> SMDMPVERILEAELAVEPKTETYVEANMGLNPSSPN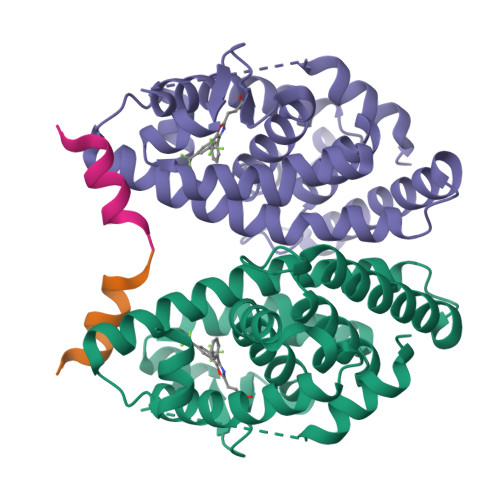DPVTNICQAADKQLFTLVEWAKRIPHFSELPLDDQVILLRAGWNELLIASFSHRSIAVKDGILLATGLHVHRNSAHSAGVGAIFDRVLTELVSKMRDMQMDKTELGCLRAIVLFNPDSKGLSNPAEVEALREKVYASLEAYCKHKYPEQPGRFAKLLLRLPALRSIGLKCLEHLFFFKLIGDTPIDTFLMEMLE;> KHKILHRLLQDSSY>[8x]GSVAVEDQPDVSAVLSAYNQQGDPTMYEEYYSGLKHFIECSLDCHRAELSQLFYPLFV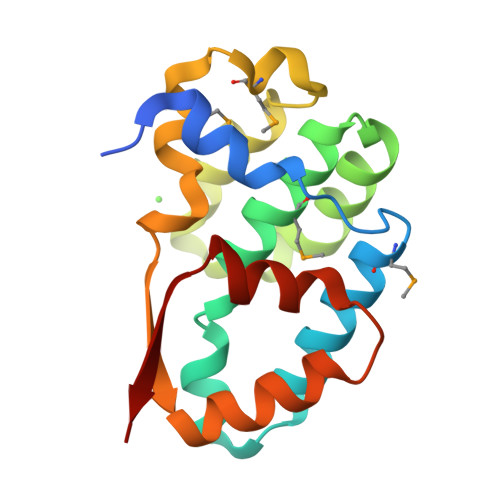HMYLELVYNQHENEAKSFFEKFHGDQECYYQDDLRVLSSLTKKEHMKGNETMLDFRTSKFVLRISRDSYQLLKRHLQEKQNNQIWNIVQEHLYIDIFD> MARSRRRMSKRSSRRSFRKYAKTHKRNFKAR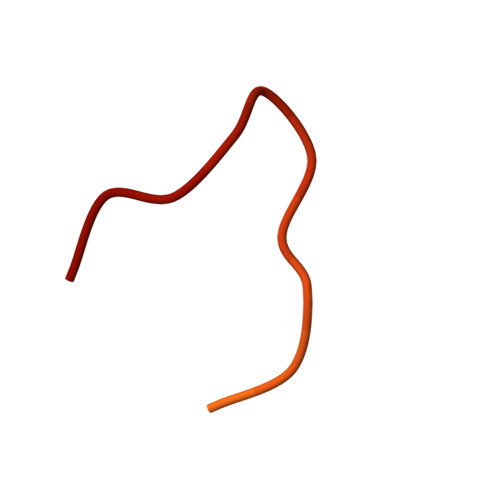SMRGGIRL>MSLWRQTPDLEQLNASQKNSIGDLLGIRFEAFDDESLTASMPVDSRTHAPFGLLHGGASVVLAES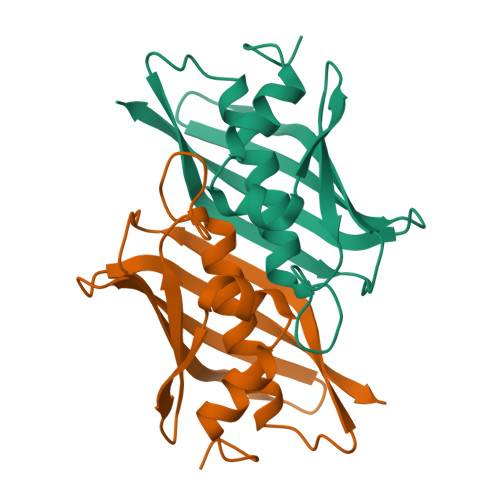LGSMASYLCVDTSQYYCVGLEVNANHLRGLRSGRVTAVARAIHLGRTTHVWDIRLSGDDGKPSCIARLTMAVVPLAGRALEHHHHHH[6x]> GHHHHHHGENLYFQGASLTEIEHLVQSVCKSYRETCQLRLEDLLRQRSNIFSREEVTGYQRKSMWEMWERCAHHLTEAIQYVVEFAKRLSGFMELCQNDQIVLLKAGAMEVVLVRMCRAYNADNRTVFFEGKYGGMELFRALGCSELISSIFDFSHSLSALHFSEDEIALYTALVLINAHRPGLQEKRKVEQLQYNLELAFHHHLCKTH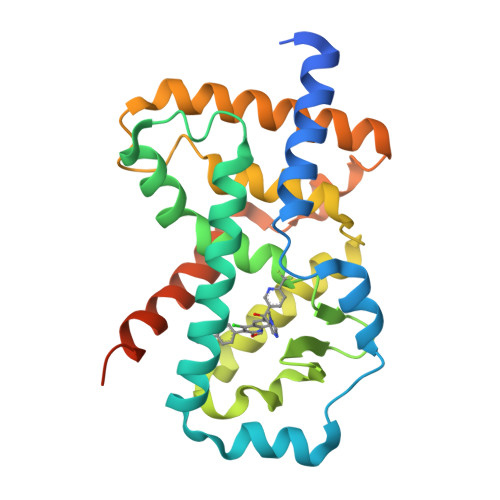RQSILAKLPPKGKLRSLCSQHVERLQIFQHLHPIVVQAAFPPLYKELFS>MGSSHHHHHHSQDPMTQNADQYRVRKEPYYRAVQDEIELYRAGYEARIPMMLKGPTGCGKSRFVEHMAWKLNRPLITIACNEDMTASDLVGRYLLDKDGTRWQDGPLTVAARIGAICYLDEIVEARQDTIVVIHPLTDHRRVLPLEKKGELVEAHPDFQIVISYNPGYQSLMKDLKQSTKQRFGALDFDYPKPDIEAEIVSHEAGVDKDTAEKLVQIAQKARNLKGHGLDEGLSTRLLVYAGKLIAKGVDARAACTMTLVNPITDDVDMRDALDTVVKTFF[2x]

Another member of the expanded α-carboxysome locus is CbbQ, a member of the AAA+ superfamily proteins (ATPases Associated with diverse cellular Activities), which are found across all kingdoms of life and fulfill a variety of functions, mostly involved in ATP-driven dissociation, unfolding and remodeling of macromolecules. Here we report the characterization of the CbbQ ortholog that is associated with the α-carboxysome locus of H. nea (Hneap_0905). We have determined the structure of CsoCbbQ, a AAA+ ATPase protein in its hexameric, nucleotide-bound form and show that it is an active ATPase. Our results implicate CsoCbbQ as a component of the assembled carboxysome, where it is tightly associated with the shell.

Hexa-histidine-tagged H. nea CsoCbbQ (Hneap_0905) was purified by affinity chromatography and crystallized with ATP in the mother liquor by vapor diffusion in sitting drops. Native data diffracting to 2.8 Å and belonging to space group H3 were collected. There are two CsoCbbQ molecules per asymmetric unit; expansion of crystal symmetry generates the full hexamer, consistent with the biologically active form of most AAA+ proteins and the size exclusion data. One molecule of ADP is bound to each monomer, indicating that the ATP is hydrolyzed during crystallization. The two chains in the asymmetric unit align only moderately well (1.2 Å rmsd over all Cα atoms) with large differences observed in the C-terminal α-helices 8 and 9 (shifted by 3–4 Å) and with electron density for some loop regions missing in chain A. The differences observed could be explained by the inherent flexibility of the chains needed for the conformational changes coupled with ATP hydrolysis, which are typically transmitted to other proteins from AAA+ domain proteins. Structurally, CsoCbbQ consists of the N-terminal P-loop NTPase domain (residues 1-175) characteristic of all AAA+ family proteins, comprising a beta sheet between two sets of α-helices. The C-terminal domain (residues 176–270), the CbbQ-specific portion of the primary structure, forms a five-helix bundle that extends from the NTPase domain. The CbbQ domain contributes only one residue, the conserved arginine finger residue R168, to the active site. Within the hexameric assembly, the majority of the CbbQ-specific domain is found on one surface of the hexamer, as a result this face of the hexamer is concave. The pronounced hexagonal profile of CsoCbbQ is distinct from that of other structurally characterized AAA+ family members, which typically display a star-shaped outline31. This hexagonal profile of CsoCbbQ is a result of the gaps in the hexamer formed by the NTPase domain being filled by the five-helix bundles of each protomer.> VNSSVEERGFLTIFEDVSGFGAWHRRWCVLSGNCISYWTYPDDEKRKNPIGRINLANCTSRQIEPANREFCARRNTFELITVRPQREDDRETLVSQCRDTLC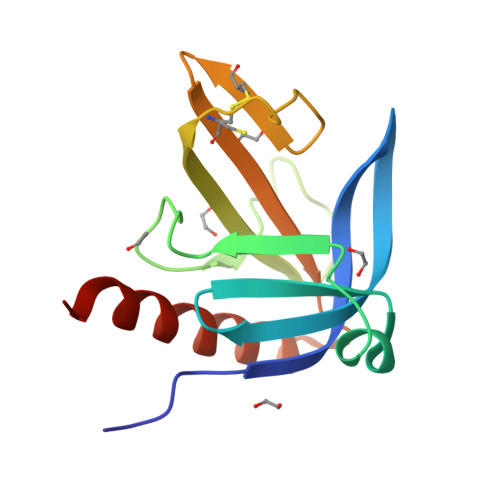VTKNWLSADTKEERDLWMQKLNQVLVDIRLWQ Here, X-ray crystallography, site-directed mutagenesis and enzymatic activity data are used to define the three-dimensional structure, acceptor/donor substrate binding, membrane binding and catalytic mechanism of PatA from M. smegmatis. PatA catalyses an essential step in the biosynthesis of PIMs in M. tuberculosis. The enzyme transfers a palmitoyl moiety from palmitoyl–CoA to the 6-position of the Manp ring linked to 2-position of myo-inositol in PIM1 or PIM2. Our results reveal that the enzyme has an α/β architecture and shares with other important eukaryotic/prokaryotic acyltransferases an acid/base catalytic mechanism involving conserved histidine and aspartic/glutamic acid residues.

The crystal structure of PatA from M. smegmatis was solved using single-wavelength anomalous dispersion with a K2PtCl4 derivative at 2.06 Å resolution in C 2 space group (PatA–C16-1). We have decided to use the PatA–C16-1 crystal form for our description since it displays the highest resolution. The high quality of the electron density maps allowed the trace of residues 41 to 302 (PatA–C16-1), 48 to 295 (PatA–C16-2) and 48 to 303 (PatA–C16-3). Strikingly, one molecule of palmitic acid was unambiguously identified in the difference electron density maps of PatA–C16-1, PatA–C16-2 and PatA–C16-3 crystal structures. We believe that acyl molecule is associated to the enzyme due to the hydrolysis of palmitoyl–CoA during the isolation and purification of PatA from M. smegmatis mc2155. The acyl chain is deeply buried into the hydrophobic pocket, and oriented with the carboxylate group facing the groove and the acyl tail extending into the globular core of the monomer. Interestingly, the comparison of the three crystal structures revealed conformational flexibility in the carboxylate moiety of the palmitate, located in close proximity with the lateral chain of H126. In all crystal structures of palmitoyl–PatA and PatA–S-C16CoA complexes, the carboxylate OE2 oxygen atom of E200 was found at 2.8 Å of the ND1 nitrogen atom of the aromatic imidazole ring of the invariant H126. It is worth noting that when the individual palmitate molecules observed in the three crystal structures of palmitoyl–PatA were superimposed, they showed important structural flexibility at the carboxylate region, suggesting that the carboxylate group is not in a catalytically competent position in the crystal structures. Our binary complexes correspond most likely to the hydrolysis reaction product of palmitoyl–CoA, thus one of the oxygen atoms found in the palmitate that interacts with H126 most likely come from a water molecule activated by H126.

>[2x]MPEVVFGSVTDLGYAAGWRLVRAMPEAMAQGVFGAGARYAARNGGPEQLRRNLARVVGKPPADVPDDLIRASLASYARYWREAFRLPAMDHGRLGEQLDVIDIDHLWSALDAGRGAVLALPHSGNWDMAGVWLVQNYGPFTTVAERLKPESLYRRFVEYRESLGFEVLPLTGGERPPFEVLAERLTDNRPICLMAERDLTRSGVQVDFFGEATRMPAGPAKLAIETGAALFPVHCWFEGDGWGMRVYPELDTSSGDVTAITQALADRFAANIATYPADWHMLQPQWIADLSDERRARLGTSRHHHHHH> GPGSDSKPVFVKVPEDQTGLSGGVASFVCQATGEPKPRITWMKKGKKVSSQRFEVIEFDDGAGSVLRIQPLRVQRDEAIYECTATNSLGEINTSAKLSVLEEDQLPSGFPTIDMGPQLKVVEKG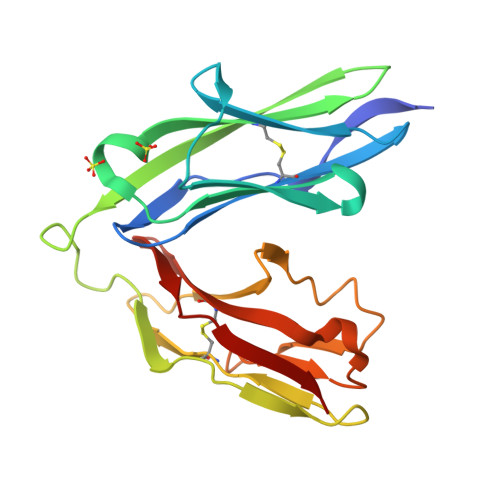RTATMLCAAGGNPDPEISWFKDFLPVDPAASNGRIKQLRSGALQIESSEESDQGKYECVATNSAGTRYSAPANLYVR> REQVKDSNGNPVKRGAKYFIQPAKSNGGGL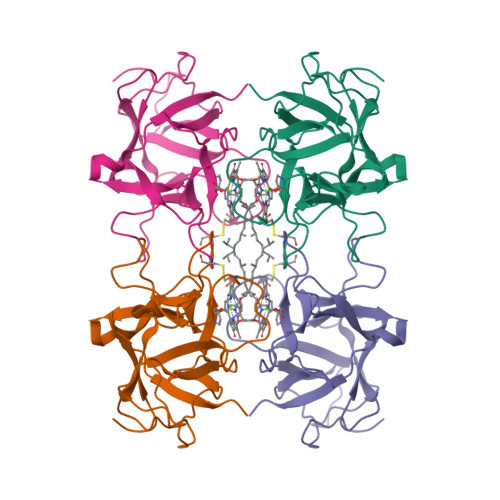VPAAINILPFCPLGITQTLLPYQPGLPVSFGYEPVIVGTDYIYTSTTINIEFRSEIWPVCNELSKLWAVDVSSSAAKEPAIIIGGERTAPNSLFKIEEATGAHTYKLTTSSGTVGTIPGPWLGAPQLIATNDDAKTLFVKFVKVDDDAT> ESWETLEADLIELSQLVTDFSLLVNSQQEKIDSIADHVNSAAVNVEE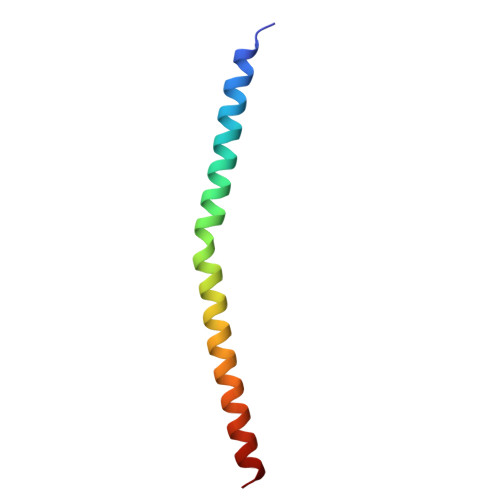GTKNLGKAAKY>RKKVRKAVIPAAGLGTRFLPATKAQPKEMLPIVDKPAIQYIVEEAAESGIEDILIITGRNKRSIEDHFDRSAELEFNLREKGKTETLKEMQQIADLANIHYIRQKEPLGLGHAVLCAEHFIGDEPFAVLLGDDIMVSETPALRQLMDVYDVYGTEVVGVQSVLPEDVSKYGIINTSGSQGHVYEVNDLVEKPSPEEAPSEIAVMGRYVLNSSIFSVLKTIGRGAGNEIQLTDALREVCRKEPIHARLLEGNRYDIGDKLGCFKASTEIGLMRPEMRSQLLAYLEDVIKRE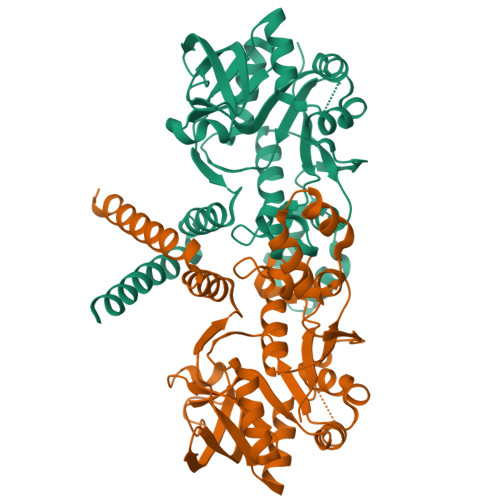TKEMLR[2x]> MKYGVYFAYWEDSWDVDFEKYVRKVKKLGLDILEVAALGLVNLPEQKLERLKQLAEQHDIILTAGIGLPKEYDVSSTDKTVRRNGITFVKKVMDAMHQAGIHRIGGTVYSYWPVDYSGPFDKPAARKHSIESVRELAEYARQYNITLLIETLNRFEQFLLNDAEEAVAYVKEVNKPNVKVMLDTFHMNIEEDHIADAIRYTGDHLGQLHIGEANRKVPGKGSMPWTEIGQALKDIRYDGYVV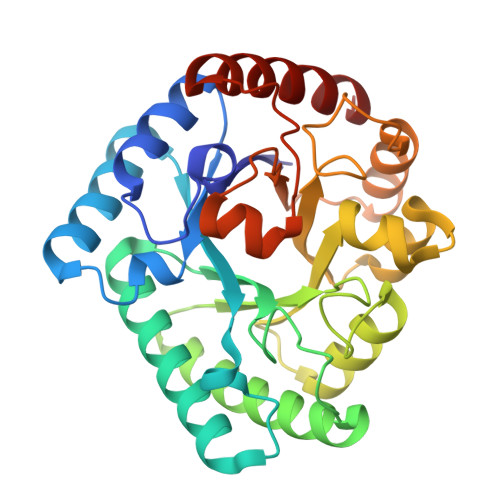MEPFVKTGGQVGRDIKLWRDLSGNATEEQLDRELAESLEFVKAAFGE>MAYPGHPGAGGGYYPGGYGGAPGGPAFPGQTQDPLYGYFAAVAGQDGQIDADELQRCLTQSGIAGGYKPFNLETCRLMVSMLDRDMSGTMGFNEFKELWAVLNGWRQHFISLDTDRSGTVDPQELQKALTTMGFRLSPQAVNSIAKRYSTNGKITFDDYIACCVKLRAL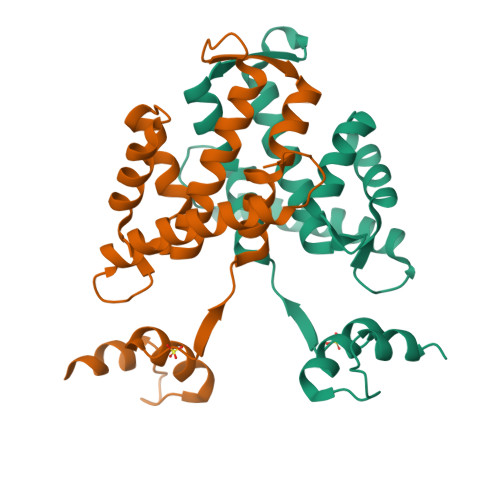TDSFRRRDTAQQGVVNFPYDDFIQCVMSV[4x]>[2x]MATSLNTIDIQGDILVGMHKQKQLFYFFAINDPATFKTHLASDIAPVVASVTQLSNVATQPLVALNIAFSNTGLLALGVTDNLGDSLFANGQAKDATSFKESTSSWVPQFAGTGIHGVIILASDTTDLIDQQVASIESTFGSSISKLYSLSASIRPGNEAGHEMFGFLDGIAQPAINGFNTPLPGQNIVDAGVIITGATNDPITRPSWAVGGSFLAFRQLEQLVPEFNKYLLDNAPAGSGSLQARADLLGARMVGRWKSGAPIDLTPTADDPALGADAQRNNNFTYSHAGFDLGSDQSHCPFSAHIRKTRPRADLGGSLTPPNLSAGANSIMRSGIPYGPEVTSAESASNTTTQERGLAFVAYQAQLSQGFHFLQQTSADNANFPPGKTPATVGLDPIIGQNNGQPRVVNGLLPSNSSASLSIPQFVVSHGGEYFFSPPISAIGGRLSA

DyPs (dye-decolorizing peroxidases) (EC 1.11.1.19) represent a new family of haem peroxidases widespread in bacteria, archaea, fungi and other micro-organisms. In the present study, we expressed A. auricula-judae DyP in E. coli, solved the crystal structure of the recombinant enzyme and several site-directed variants, and used PELE (Protein Energy Landscape Exploration) to describe the binding of its typical substrate RB19. The DyP structure is formed by two domains, each of them including an antiparallel four-stranded large β-sheet and two or three helices resulting in a ferredoxin-like fold (plus two additional β-strands). In spite of the obvious similarity between the two domains, only the C-terminal domain harbours a haem cofactor.

Aromatic residues were changed to serine in the simple W377S, Y147S and Y337S variants (the latter with low refolding yield). Moreover, most of the variants show crystal structures largely superimposable with that of WT DyP, except for the mutated residues. The proof for Trp-377 being involved in the mixed protein radical was provided by the W377S variant. In the high-resolution narrow scan of its 9 GHz EPR spectrum (top), the tryptophanyl contribution observed for WT DyP completely disappeared (the spectrum of the W377S/Y147S variant, not shown, being nearly superimposable). The W377S spectrum (top) shows a single line with hyperfine resolution at g=2.0046(2). Simulation of this spectrum at X-band (bottom) confirmed that it corresponds to a tyrosine phenoxyl radical. As a main conclusion, Trp-377 appears responsible for the high-turnover catalytic site, since its substitution (W377S variant) completely prevented high-turnover oxidation of RB19 and DMP (and decreased over 40-fold the catalytic efficiency of high-turnover ABTS oxidation). Site-directed mutagenesis showed that high-turnover oxidation of RB19 and other substrates by DyP takes place at the same tryptophan residue (Trp-377), identified previously as forming a protein radical. Acidic pH optima were already reported for A. auricula-judae DyP, and are also typical of lignin-degrading peroxidases (LiP and VP). It is interesting that a delay period was not observed in oxidation reactions with WT DyP, and its W377S variant described below, which showed identical reaction traces and MALDI–TOF molecular masses with/without treatment with VA and H2O2.>VITLPKLKYALNALSPHISEETL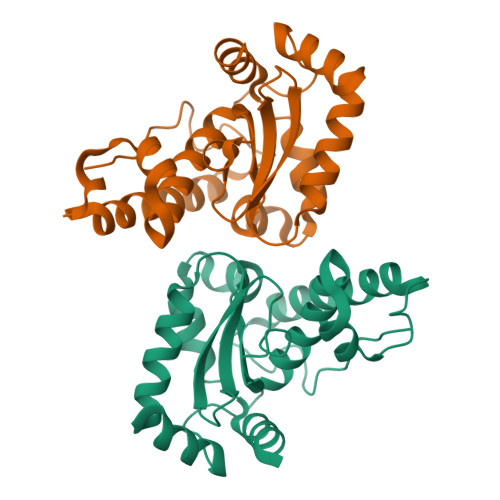NFHYNKHHAGYVNKLNTLIKDTPFAEKSLLDIVKESSGAIFNNAAQIWNHTFYWDSMGPDCGGEPHGEIKEKIQEDFGSFNNFKEQFSNILCGHFGSGWGWLALNNNNKLVILQTHDAGNPIKDNTGIPILTCDIWEHAYYIDYRNDRASYVKAWWNLVNWNFANENLKKAMKK[2x]5-methylphenazin-1(5H)-one | C13 H10 N2 O | 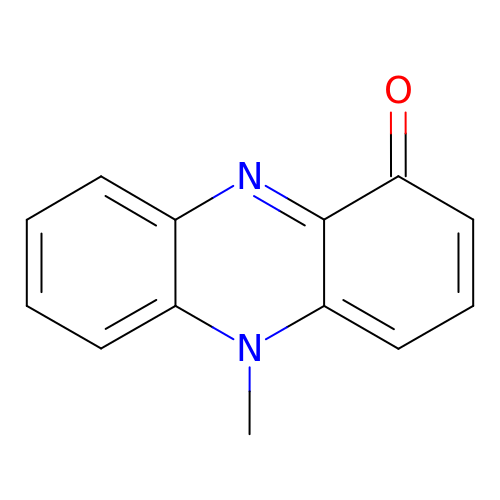YNCMLFHHXWETLD-UHFFFAOYSA-N> MDLVEEILRLKEERNAIILAHNYQLPEVQDIADFIGDSLELARRATRVDADVIVFAGVDFMAETAKILNPDKVVLIPSREATCAMANMLKVEHILEAKRKYPNAPVVLYVNSTAEAKAYADVTVTSANAVEVVKKLDSDVVIFGPDKNLAHYVAKMTGKKIIPVPSKGHCYVH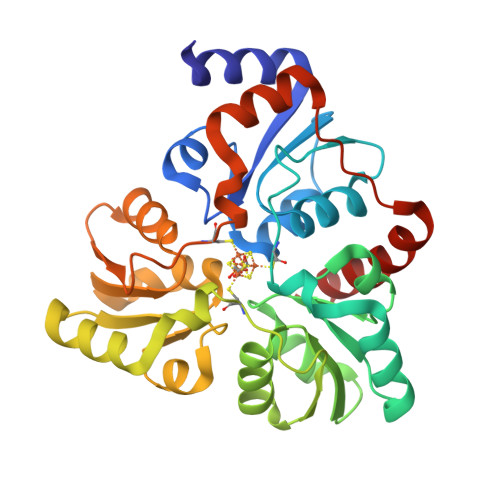QKFTLDDVERAKKLHPNAKLMIHPECIPEVQEKADIIASTGGMIKRACEWDEWVVFTEREMVYRLRKLYPQKKFYPAREDAFCIGMKAITLKNIYESLKDMKYKVEVPEEIARKARKAIERMLEMSK>MPQEARTPQQQVTADEVGDWYDKFGE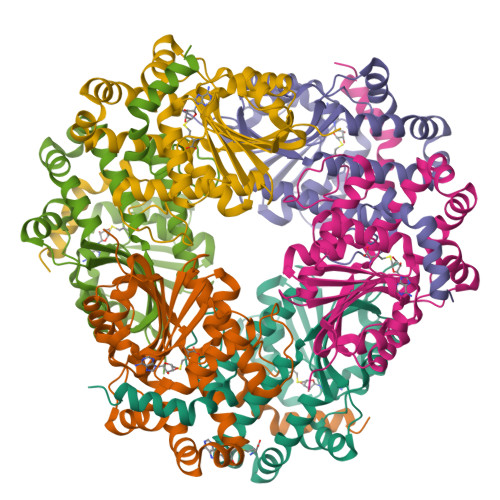VYHLTLGESVHCGLWFPPDAPVPQDMELVTMSSQAQDRYTDYLIETLDPKAGQHLLDIGCGTGRTALKAARQRGIAVTGVAVSKEQIAAANRLAAGHGLTERLTFEVADAMRLPYEDESFDCAWAIESLCHMDRAKALGEAWRVLKPGGDLLVLESVVTEELTEPETALFETLYAANVPPRLGEFFDIVSGAGFHTLSLKDLSANLAMTMNVFALGVYSRRAEFTERFGAEFVDGLLAGLGSAQETLIRKTRFFMATLRKPAVLEHHHHHH[18x]> GPGSKHNVKLSSVPSLLHGLYLYKHQQYQKAQEIFNKILEKQPQNAYLNFRYGMALYKDKKWDEANHFIQKAVELAPEKEAWKKQLATTERYKHDSSKVKVAENKKKLEANPNSPEYIWEYAISLIDSKQYWLAQFQLEKYIELKPNSEQAFHQLGIVSEKLANYEQAFIYFQKASQFAPLNRNYKYRMGYNLEKLGKLNEAQKCYSLVIDMSHPTDEVAQFGIGALHAKRGLWDMALSAYLQHQIQSNSQNPQLYYRIGIAYERLYQWTKSATTFEQAIILSEIMNANWCFKCGQAYERAENFEKSAEFYQEAVKRSDNYNDYWWYRLALMLEKLGKYEQSVVAFQNSRRRKLAYAVNPKDVIKHKEEEFLSYYTEYYETLELDEKLVLIESFFGGNISCNPYAILSYMLENNYDYTYVVVIKDGTVIPDNLKFNRNIIFIKRGSDAYLRYLCTAKYLINNVSFPYYFIRKEGQVYLNTWHGTPMKTLGKDIKSPFMDHANVSRNFLQATHIISPNRHTTDVILEQYDVKDLFSGKLAETGYPRIDLSFNLTDKRRNEIAEKLGFSNNKPVVFYAPTWRGTSQSKDFDTSKLQYDLRKLKSNKYNLIFRGHHLVEQLLETINLDVTVAPKDIDSNELLGFCDLLITDYSSIIYDFLALSKPAISYIYDYEEYDAERGLYLKPTEMSGTVCTTITDVKKTILEHISSGKSNVSEQDIQKYSYLDDGQATKRTVEFMLDKDDSCIYKYERRKSDVFFEGPFIPNGISRSFLNLMASIKDSGKNITLLINGSDIAQDQKRLEEFNNLPSNITVLSRVGRTPMTLEELWVRNKFEETYQIYSESFTNTLLKVYKREVRRLLGNSSFDNAIHFEGYSLFWVLLFSQINAKKHIIYQHNDKYKEWKGRFPYLEGVFNSYVFFDQIVSVSEKTMENNILNLSKEFNIPEIKFTFCNNPINIQQILSSAEENIEMESEFTLFNGQKFINIGRMSHEKDQLKLIEAFYEAKKAHVNIRLFILGDGVLKQDLINKIKDLSLEDSVYLLGQKKNPFPYLKQADVFILSSNHEGQPMVLLESLTLGTPIIATDIVGNRSILGENYGTLVENNKDGLVQGINAYMEKGGRKDKFDPYEYQNDAMAKFYSLLANLEHHHHHH

Capsules are long-chain carbohydrate polymers that envelop the surfaces of many bacteria, protecting them from host immune responses. Using Actinobacillus pleuropneumoniae as an example, we demonstrate that CpsA and CpsC generate a poly(glycerol-3-phosphate) linker to connect the glycolipid with capsules containing poly(galactosylglycerol-phosphate) backbones. We reconstruct the entire capsule biosynthesis pathway in A. pleuropneumoniae serotypes 3 and 7, solve the X-ray crystal structure of the capsule polymerase CpsD, identify its tetratricopeptide repeat domain as essential for elongating poly(glycerol-3-phosphate) and show that CpsA and CpsC stimulate CpsD to produce longer polymers. The polymer backbones of App3 and App7 are composed of related poly(glycosylglycerol phosphate) structures ([→4)-α-Gal-(1→2)-Gro-(3-PO4−] and [→3)-α-Gal-(1→1)-Gro-(3-PO4−], respectively) and both Cps3D and Cps7D require the alternating action of a CgoT and a CgaT domain for the transfer of Gro3P and Gal, respectively.

Because attempts to crystallize Cps7D failed, we solved the crystal structure of the homologous capsule polymerase Cps3D from App3 (38% sequence identity; A0A2S0ETM3; 1138 residues). The crystal structure of Cps3D in its unliganded form was solved by molecular replacement methods to a maximum resolution of 3.0 Å. Cps3D (maltose-binding protein (MBP)-Cps3D2–1138-His6; Supplementary Figs. 1 and 8) crystallized in the P 3 2 1 space group with one molecule in the asymmetric unit, and the electron density maps allowed us to trace residues 100 to 1,145. Cps3D is a multi-modular enzyme composed of three regions from the N- to the C-terminus: (1) a TPR domain (residues 100–357; orange), (2) a CgoT domain (residue 358–736; yellow) and (3) a CgaT domain (residues 748–1,136; red). The Cps3D protomers build into a physiological and functional dimer (overall size ca. 170 Å × 95 Å × 70 Å). Dimerization was confirmed by size exclusion chromatography. The dimeric architecture is assembled primarily by an extensive interaction network between (1) the two TPR (α2–α15) and TPR′ domains and (2) the TPR domain and the N-terminal domain of CgaT′ (CgaT′-NT). CgoT adopts the typical GT-B fold of glycosyltransferases consisting of two Rossmann-fold domains. Similarly, CgaT displays a GT-B fold. The CgoT and CgaT active sites are located buried between the corresponding two Rossmann-fold domains, including the essential residues for catalytic activities.>[3x]MTPLLELKDIRRSYPAGDEQVEVLKGISLDIYAGEMVAIVGASGSGKSTLMNILGCLDKATSGTYRVA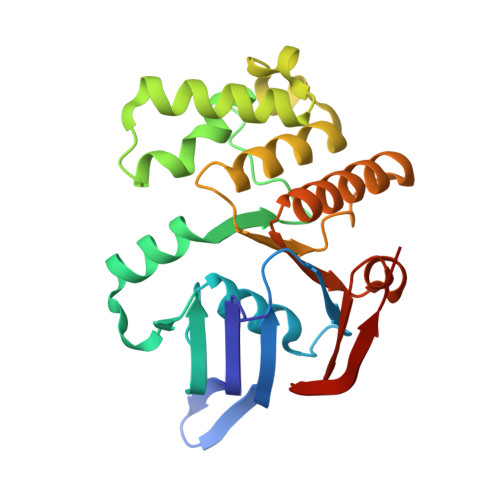GQDVATLDADALAQLRREHFGFIFQRYHLLSHLTAEQNVEVPAVYAGLERKQRLLRAQELLQRLGLEDRTEYYPAQLSGGQQQRVSIARALMNGGQVILADEPTGALDSHSGEEVMAILHQLRDRGHTVIIVTHDPQVAAQAERVIEIRDGEIVRLEHHHHHH> MPYHEFEVSKCIPERREHAVMKAAGEDLTSCLPKGYLNTIPGTISERGCAYCGAKHVIGTPMKDVIHISHGPNGCTYDTWQTKRYISDNDNFQLKYTFATDVKEKHV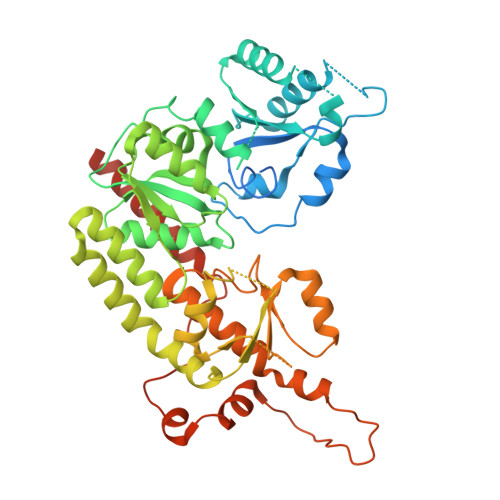VFGAEGLLKKSMHEAFDAFPNIKRMTVYQTCTTALIGDDVDAIAKEVMEERGDVDVFVCNSPGFAGPSQSGGHHKINIAWLNQKVGTVEPDYLGEHVINYVGEYNIQGDQEVMIDYFNRMGIQVLSTFTGNGSYDSLRMMHRAHLNVLECARSAEYICDELRARYGIPRLDIDGFGFEPLANSLRKVALFFGIEDKAEAIIAEEYAKWKPQLDWYKERLKGKKVCLWPGGSKLWHWAHAIEEEMGLKVVSVYTKFGHQGDMEKGVSRCGEGALAIDDPNELESVEAIEMLKPDIIFTGKRPGEFVKKHGVPYLNAHAYHNGPYKGFEGWVRFARDIYNAIYSPMRQLAALDISAPDAAITSGFRTAKMNADLTVSDEVKFSEVLHEYTGKYDSIAEIRARNQAYAAEQKALRDAVQPAAEWSHPQFEK>MDSDTDTDSGPVVATTKLVTFLQRVQHTALRSYPKKQTPDPKSYIDLSLKRPYSLSTIESAFDDLTSE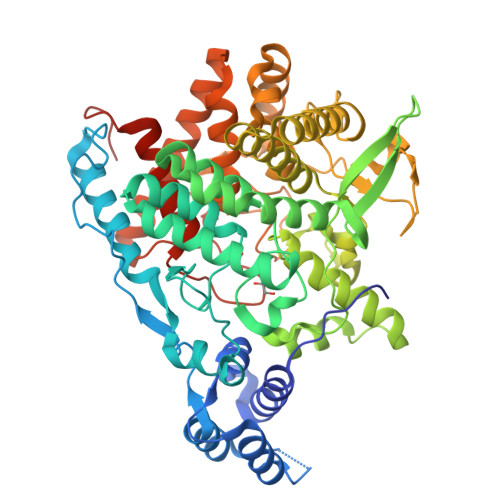SHDQPVPVETLEKFVKEYFDGAGEDLLHHEPVDFVSDPSGFLSNVENEEVREWAREVHGLWRNLSCRVSDSVRESADRHTLLPLPEPVIIPGSRFREVYYWDSYWVIKGLMTSQMFTTAKGLVTNLMSLVETYGYALNGARAYYTNRSQPPLLSSMVYEIYNVTKDEELVRKAIPLLLKEYEFWNSGKHKVVIRDANGYDHVLSRYYAMWNKPRPESSVFDEESASGFSTMLEKQRFHRDIATAAESGCAFSTRWMRDPPNFTTMATTSVVPVDLNVFLLKMELDIAFMMKVSGDQNGSDRFVKASKAREKAFQTVFWNEKAGQWLDYWLSSSGEESETWKAENQNTNVFASNFAPIWINSINSDENLVKKVVTALKNSGLIAPAGILTSLTNSGQQWDSPNGWAPQQEMIVTGLGRSSVKEAKEMAEDIARRWIKSNYLVYKKSGTIHEKLKVTELGEYGGGGEYMPQTGFGWSNGVILAFLEEYGWPSHLSIEALEHHHHHH[4x]> GSHTAEEDMEDDTSWRSEATFQFTVERFSRLSESVLSPPCFVRNLPWKIMVMPRFYPDRPHQKSVGFFLQC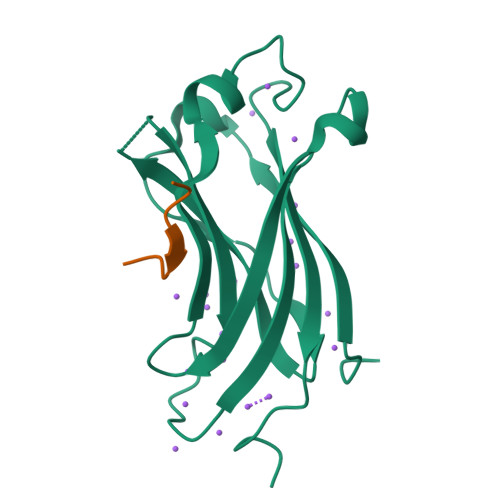NAESDSTSWSCHAQAVLKIINYRDDEKSFSRRISHLFFHKENDWGFSNFMAWSEVTDPEKGFIDDDKVTFEVFVQADAPHGVAW;> DPGEGPSTGP1,2-CIS-1-HYDROXY-2,7-DIAMINO-MITOSENE 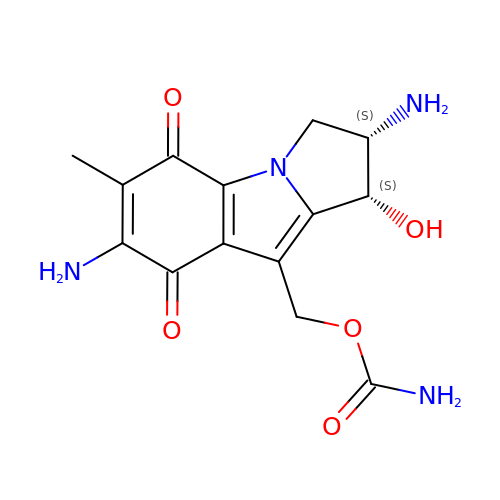| C14 H16 N4 O5 | XNHZZRIKMUCTHU-QTTZVWFDSA-N>[2x]MDPMQKRAIYPGTFDPITNGHIDIVTRATQMFDHVILAIAASPSKKPMFTLEERVALAQQATAHLGNVEVVGFSDLMANFARNQHATVLIRGLRAVADFEYEMQLAHM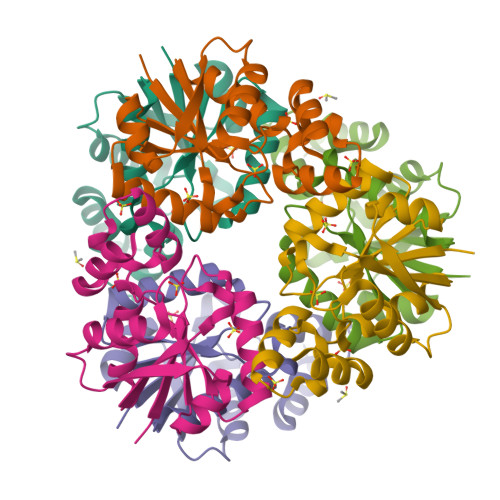NRHLMPELESVFLMPSKEWSFISSSLVKEVARHQGDVTHFLPENVHQALMAKLAVDHHHHHH> APADPGKAGVPGVAAPGAPAAAPPAKEIPEVLVDPRSRRRYVRGRFLGKGGFAKCFEISDADTKEVFAGKIVPKSLLLKPHQREKMSMEISIHRSLAHQHVVGFHGFFEDNDFVFVVLELCRRRSLLELHKRRKALTEPE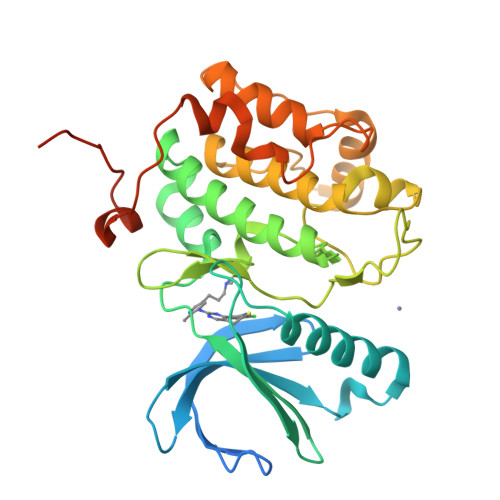ARYYLRQIVLGCQYLHRNRVIHRDLKLGNLFLNEDLEVKIGDFGLATKVEYDGERKKVLCGTPNYIAPEVLSKKGHSFEVDVWSIGCIMYTLLVGKPPFETSCLKETYLRIKKNEYSIPKHINPVAASLIQKMLQTDPTARPTINELLNDEFFTSGYIPARLPITCLTIPPRFSIAPSSLDPSNRKPLTVLNK> MVYHLFERICNPDNFKLSGEAARVRTLIAAGFSKEEAEQVAWLQNHQVNGKILGLFTGGFALYCCNNYFHYFERYFPRLRYQPFTKFLAQAATVYFFFKIGDYYFTSRRYGSNDARMNGLMYSNTYYSTNKEALIQNFEPLNRKFTEEEVEQFLRNEGRSQEEKRNWIYNPHIHGSTEGEWKADIHEKFDSGKAPWEREHVKAKILETNKAKIDAG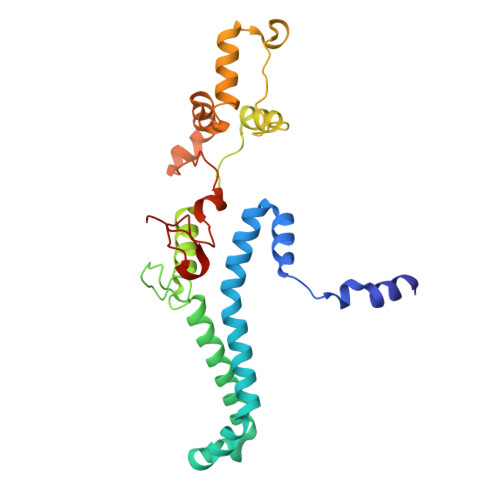EEIQLKPFKTLNHLDKTGLLHRLHPFIWTNNWTLLG>GMLTGKHVVIIGGDARQLEIIRKLSTFDAKISLVGFDQLDDGFIGVTKMRIDEVDWNTVDAILLPISGTNEAGKVDTIFSNESIVLTEEMIEKTPNHCVVYSGISNTYLNQCMKKTNRTLVKLMERDDIAIYNSIPTAEGTIMMAIQHTDFTIHGANVAVLGLGRVGMSVARKFAALGAKVKVGARESDLLARIAEMGMEPFHISKAAQELRDVDVCINTIPALVVTANVLAEMPSHTFVIDLASKPGGTDFRY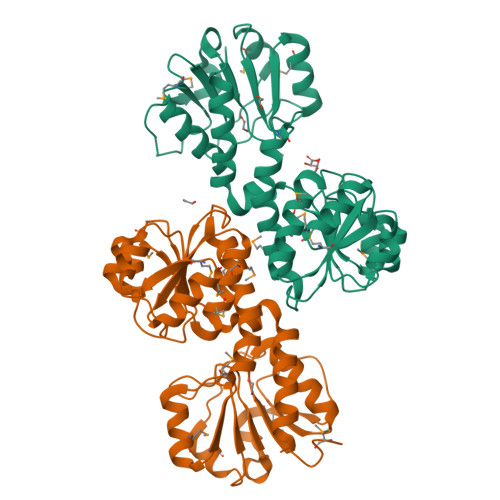AEKRGIKALLVPGLPGIVAPKTAGRILADVLVKLLAEPS[4x]>MCTGVRFSDDEGNTYFGRNLDWSFSYGETILVTPRGYHYDTVFGAGGKAKPNAVIGVGVVMADRPMY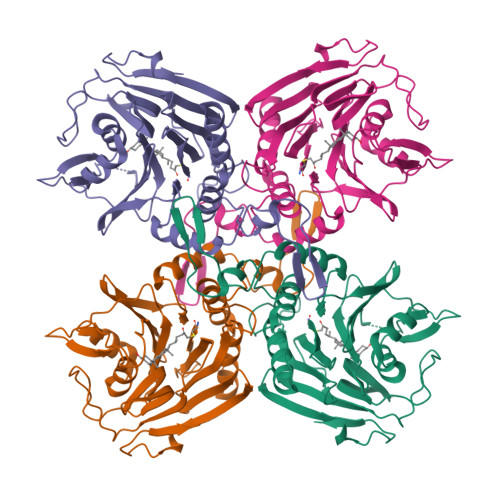FDCANEHGLAIAGLNFPGYASFVHEPVEGTENVATFEFPLWVARNFDSVDEVEETLRNVTLVSQIVPGQQESLLHWFIGDGKRSIVVEQMADGMHVHHDDVDVLTNQPTFDFHMENLRNYMCVSNEMAEPTSWGKASLTAWGAGVGMHGIPGDVSSPSRFVRVAYTNAHYPQQNDEAANVSRLFHTLGSVQMVDGMAKMGDGQFERTLFTSGYSSKTNTYYMNTYDDPAIRSYAMADYDMDSSELISVAR[2x]N-METHYLMESOPORPHYRIN | C35 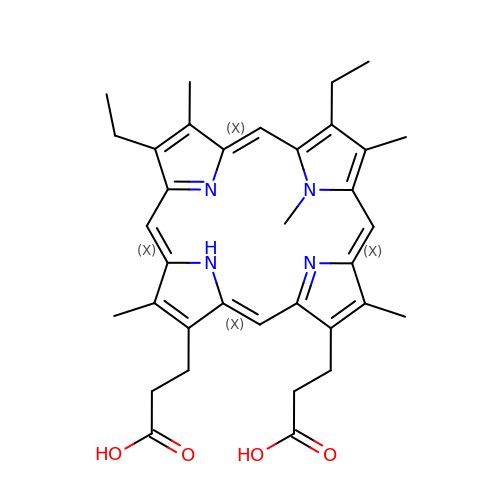H40 N4 O4 | YNWHQWMCLCANDI-YIYRCNGCSA-N>CCTGCGCAGG[2x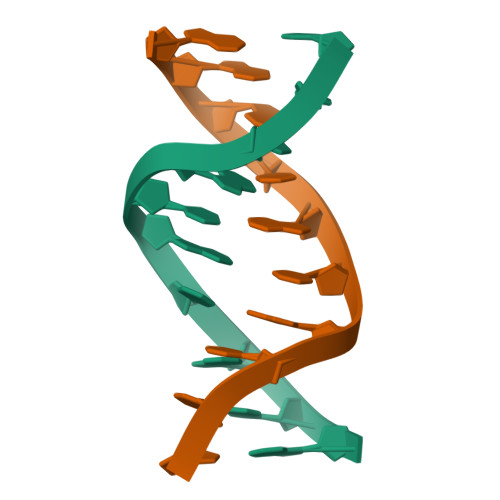]>[2x]MITAYIALGSNLNTPVEQLHAALKAISQLSNTHLVTTSSFYKSKPLGPQDQPDYVNAVAKIETELSPLKLLDELQRIENEQGRVRLRRWGERTLDLDILLYGNEIIQNERLTIPHYD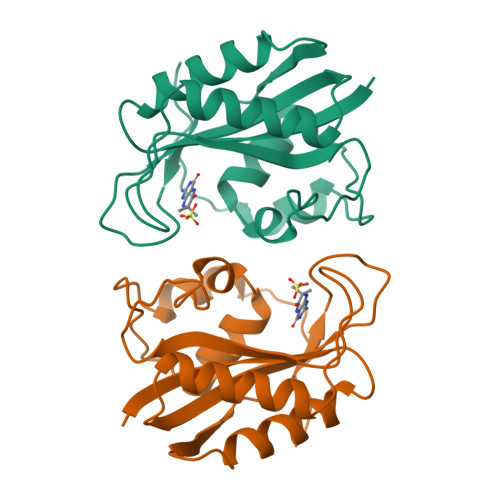MHNREFVIVPLFEIASDLVLPNSQIITELVKQFADHKMIKLNP>[2x]MATKKATMIIEKDFKIAEIDKRIYGSFIEHLGRAVYGGIYEPGHPQADENGFRQDVIELVKELQVPIIRYPGGNFV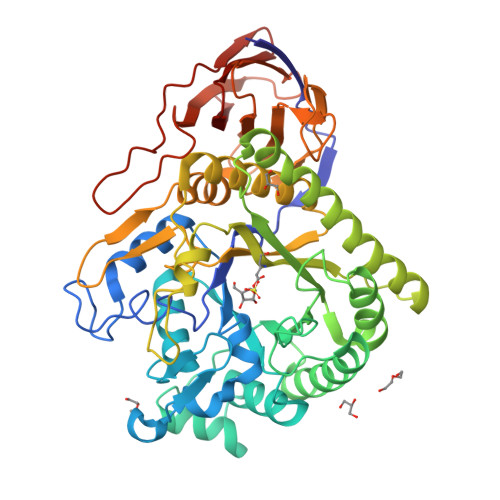SGYNWEDGVGPKEQRPRRLDLAWKSVETNEIGLNEFMDWAKMVGAEVNMAVNLGTRGIDAARNLVEYCNHPSGSYYSDLRIAHGYKEPHKIKTWCLGNEMDGPWQIGHKTAVEYGRIACEAAKVMKWVDPTIELVVCGSSNRNMPTFAEWEATVLDHTYDHVDYISLHQYYGNRDNDTANYLALSLEMDDFIRSVVAIADYVKAKKRSKKTIHLSFDEWNVWYHSNEADKLIEPWTVAPPLLEDIYNFEDALLVGCMLITLMKHADRVKIACLAQLVNVIAPIMTEKNGPAWKQTIYYPFMHASVYGRGVALHPVISSPKYDSKDFTDVPYLESIAVYNEEKEEVTIFAVNRDMEDALLLECDVRSFEDYRVIEHIVLEHDNVKQTNSAQSSPVVPHRNGDAQLSDRKVSATLPKLSWNVIRLGKR1-[4-({[6-amino-5-(4-phenoxyphenyl)pyrimidin-4-yl]amino}methyl)piperidin-1-yl]prop-2-en-1-one 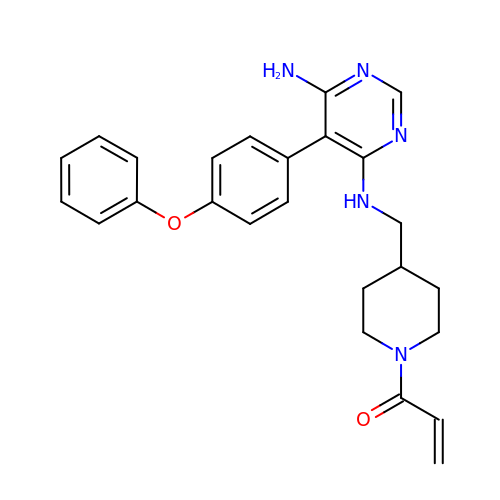| C25 H27 N5 O2 | QUIWHXQETADMGN-UHFFFAOYSA-N>SMKLDIKKTFSNRSDRVKGIDFHPTEPWVLTTLASGRVEIWNYETQVEVRSIQVTETPVRAGKFIARKNWIIVGSDDFRIRVFNYNTGEKVVDFEAHPDYIRSIAVHPTKPYVLSGSDDLTVKLWNWENNWALEQTFEGHEHFVMCVAFNPKDPSTFASGCLDRTVKVWSLGQSTPNFTLTTGQERGVNYVDYYPLPDKPYMITASDDLTIKIWDYQTKSCVATLEGHMSNVSFAVFHPTLPIIISGSEDGTLKIWNSSTYKVEKTLNVGLERSWCIATHPTGRKNYIASGFDNGFTVLSLG[2x];> GVKLHYE

Hence, this loss of critical proteins has the potential to compromise ER proteostasis and generate cellular stress. This challenge to normal metabolism is overcome by the activity of the cytosolic coatomer protein I (COPI) polymer, whose repeating unit is the coatomer, a 560 kDa complex of seven distinct gene products (α-, β-, β′-, γ-, δ-, ε-, and ζ-COPI)25–31. Overall, the coatomer functions to retrieve the escaped “client” proteins, such as type I membrane proteins, from cis-Golgi back to ER by retrograde trafficking. In particular, the S protein – a type I membrane protein – is delivered to the ERGIC from both the ER (by anterograde trafficking) and the Golgi (by retrograde trafficking)3,10–12. Here we utilize recombinant SARS-CoV-2 S proteins and tail peptides, including constructs with enhanced mimicry of the coatomer binding motif (clientized S protein), to elucidate the atomic structure of the S-coatomer interface.

Furthermore, our co-crystal structures showed that the Tyr33 side chain of β‘WD40 pushes away the Tyr1272 side chain of the S heptapeptide. This Tyr33 is replaced by a smaller His31 residue in the αWD40 domain. We hypothesized that the replacement of the bulky Tyr33 side chain with a smaller residue would allow Tyr1272 to move closer to the β‘WD40 surface, thereby further strengthening the binding between S and β‘WD40. Therefore, we generated a β‘WD40 Tyr33Ala mutant and determined its co-crystal structure with the clientized S heptapeptide at a resolution of 1.8 Å. Although the S Tyr1272 side chain was indeed closer to the mutant β‘WD40 surface by 0.8 Å, overall, the Tyr1272 side chain was still >4 Å away from the β‘WD40 surface. A BLI assay revealed this was insufficient to enhance S-β‘WD40 affinity. Moreover, this β‘WD40 Tyr33Ala mutation abolished binding to the clientized Thr1273Glu S heptapeptide, suggesting a previously unrecognized role for β‘WD40 Tyr33 in S heptapeptide binding. Moreover, β‘WD40 Tyr33 plays a critical role in stabilizing S tail binding through interactions with the tail Tyr1272 side-chain.>MALSLYEKMLHKGMIIKNSNVYEKIKEIDTIIFNKTGTLTYGTPIVTQFIGDSLSLAYAASVEALSSHPIAKAIVKYAKEQGVKILEVKDFKEISGIGVRGKISDKIIEVKKAENNNDIAVYINGEPIASFNISDVPRPNLKDYLEKLKNEGLKIIILSGDKEDKVKELSKELNIQEYYS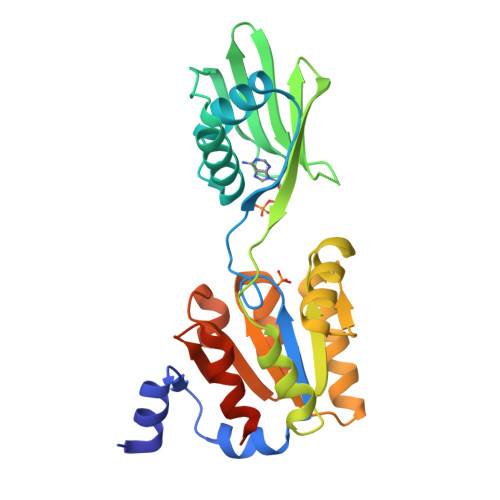NLSPEDKVRIIEKLKQNGNKVLMIGDGVNDAAALALADVSVAMGNGVDISKNVADIILVSNDIGTLLGLIKNRKRLSNAIPSN[2x]>MMSETAPLPSASSALEDKAASAPVVGIIMGSQSDWETMRHADALLTELEIPHETLIVSAHRTPDRLADYARTAAERGLNVIIAGAGGAAHLPGMCA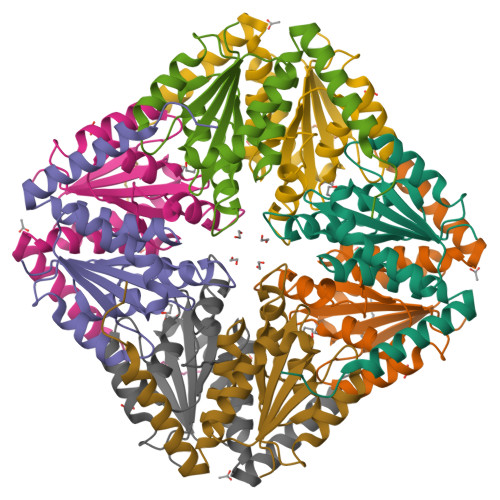AWTRLPVLGVPVESRALKGMDSLLSIVQMPGGVPVGTLAIGASGAKNAALLAASILALYNPALAARLETWRALQTASVPNSPITEDK[2x]> GMQNSQEMAITTLSLPKGGGAINGMGESVGQAGPDGMVTFSIPLPFSAGRGVAPALSLSYSSGAGNGPFGMGWQCSAMSISRRTQKGVPQYNEDDEFLSPSGEVMAIALNDSGFEDVRTANRLQGIPLPFSYKVTRYQPRLIQDFIKIEYWQPVKQTDGTPFWIIYSPDGQTHILGKNSHSRVANAENPSQIASWLLEETVTPTGEHIYYQYSGENQVNCTDAEIALHPQDSAQRYLARIDYGNISPQASLFVLDEELPNLTQWLFHLVFDYGERDISINKIPTFEGGTTGWLARPDMFSRYDFGIEIRNRRLCHQVLGFHRLEALNDRDVTDEIPVLVNRLTLDYDLNNSVSTLVAVRQVAYETDGSPITQPPLEFDYQRFDTGSIPGWQEMPQLEAFNGYQPYQMIDLYGEGTPGILYQETPGAWWYKSPQRQIGGDSNAVTYGAMKALPKIPRLQEGATLMDINGDGRLDWVITSAGVRGFHSIHSTGEWTHFTPLNTLPTEYFHPKAQLADLVGAGLSDLVLIGPKSVRLYANQQGNWAPAQDVTQAENVSLPV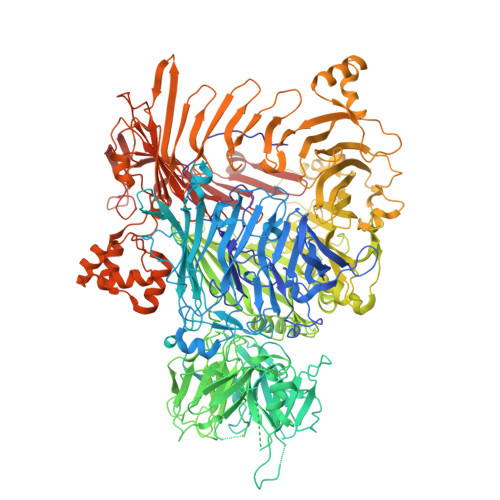IGIDSRQLVAFADMLGSGQQHLVEITADSVKCWPNMGHGRFGQPLTLEGFSQPQTSFNPDRVFLADIDGSGTNDIIYAHSECLEIYLNESGNRFSKPISLLLPDGVNFDNTCQLQAADIQGLGIASLVMTVPHMSPTHWRCDLALNKPWLLNVMNNNRGAETCLFYRSSAQFWLDEKQLVEAAGQQPECHLPFPMHLHWRSEIFDEITGNRLTQEQEYAHGSWDGQEREFRGFGRLIQRDTDGFAQGTVDIPTHPSRTVSWFATGIPEIDTTLSAEFWRGDDQAFSPFSPRFTRWENDSEAGSDVAFIPSEHDAFWLNRAMKGQLLRSELYGDDGTPEAEIPYSVTEMRHQVRALPTTDATVPSAWCSTIETRSYQYQRVAADPQCSQQVVIKADRYGSPLLSVAINYPRRKKPEKSPYPDDLPETLFDSSYDTQQQQLHLTKQQQNYFHLTNDDNWLLGLPKEQRNDGYQYDQERAPANGFTLETLIASNSLIGSNQPFTYLGQSRVAYQGGVDEQPSLQALVAYGETAILDEKTLQAFVGVLDSKTRDELLFSAGYQLAPRLFRVESEPDVWVARQGYSEFGDYSQFWRPLSQRSTLLTGKTTLKWDKHYCVVIETQDAAQLVTQARYDYRFLTPYSLTDANDNQHYVVLNPFGEVIASRFWGTEAGKDAGYSTPQAKPFVVPATIEAALALSPGIPVAHCAIFEPESWMQKLTQHDVSERMADNGTLWNALLQARFVTEDGYVCALGRRRWMARHGLSVLMLTLLAEIPRTPPHSLTITTDRYDSDDQQQLRQRILFSDGFGRLLQSAQRVEAGESWQRSEDSSLVVNVSGTPALVVTDNRWAVSGRTEYDGKGQGIRVYQPYFLDDWRYLSDDSARTDLFADTHIYDPLGREYQVITAKGYRRERQYTPWFVVNQDENDTAANLAI>MAKFFIDRPIFAWVISIFIIAAGIFGIKSLPVSQYPSVAAPTITLHAIYPGASAQVMEGSVLSVIERNMNGVEGLDYMSTSADSSGSGSVSLTFTPDTDENLAQVEVQNKLSEVLSTLPATVQQYGVTVSKARSNFLMIVMLSSDVQSTEEMNDYAQRNVVPELQRIEGVGQVRLFGAQRAM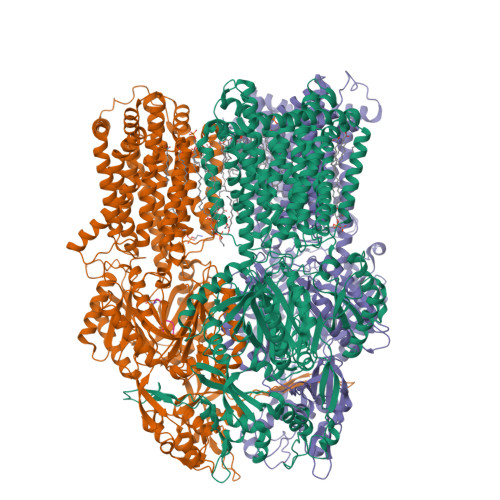RIWVDPKKLQNYNLSFADVGSALSAQNIQISAGSIGSLPAVRGQTVTATVTAQGQLGTAEEFGNVILRANTDGSNIYLKDVAKVGLGMEDYSSSTRLNGVNTTGMAVMLSNSGNAMATAKAVKERLAVLEKYFPQGMSWKTPYDTSKFVEISIEKVIHTLIEAMVLVFVVMYLFLQNIRYTLIPTIVVPISLLGGFAFISYMGMSINVLTMFAMILVIGIVVDDAIVVVENVERIMAGEGLPPKEATKKAMGQISGAVIGITAVLISVFVPLAMFSGAAGNIYKQFALTMASSIAFSAFLALTLTPALCATMLKTIPKGHHEEKKGFFGWFNKKFDSWTHGYEGRVAKVLRKTFRMMVVYIGLAVVGVFLFMRLPTSFLPTEDQGFVMVSVQLPAGATKERTDATLAQVTQLAKSIPEIENIITVSGFSFSGSGQNMAMGFAILKDWNERTASGSDAVAVAGKLTGMMMGTLKDGFGIAVVPPPILELGNGSGLSINLQDRNNTGHTALLAKRNELIQKMRASGLFDPSTVRAGGLEDSPQLKIDINRAAAAAQGVSFADIRTALASALSSSYVSDFPNQGRLQRVMVQADGDARMQPADILNLTVPNSSGIAVPLSSIATVSWQMGTEQSVRFNGYPAMELSGSPATGVSTGQAMEAVQKMVDELGSGYSLEWGGQSREEAKGGSQTIALYALAAVAVFLVLAALYESWSIPLAVLLVMPLGLAGAAAGVTGRNLFEGLLGSVPSFANDIYFQVGFVTVMGLSAKNAILIIEFAKDLQAQGKSAVEAALEAARLRFRPIIMTSFAFILGVVPLYIAGGASSASQRAIGTTVFWGMLIGTLLSVFLVPLFYVVVRKFFKETAHEHEMAVRHASKAGITGSDDKQY[3x];> CTNEDGKPC> MGSSHHHHHHSSGENLYFQGSHMTATATSAKAAAPACPRFDDPVHAAADPRVDVERITPDPVWR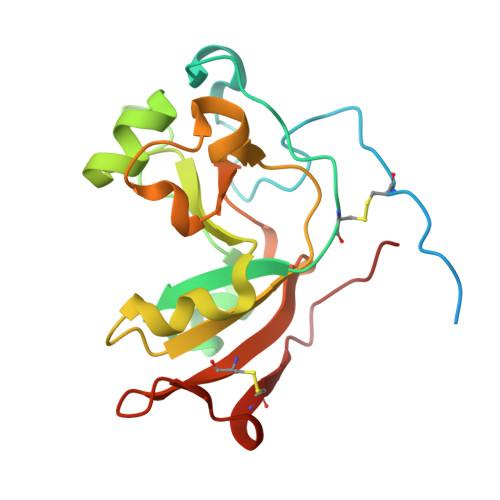TTCGTLYRSDSRGPAVVFEQGFLPKDVIDGQYDIESYVLVNQPSPYVSTTYDHDLYKTWYKSGYNYYIDAPGGVDVNKTIGDRHKAADQVEVAFPGGIRTEFVIGVCPVDKKTRTEKMSECVGNPHYEPWH>MATNFFIQPITEEAEAYYPPSVITNKRKDLGVDVYCCSDLVLQPGLNIVRLHIKVACEHMGKKCGFKIMARSSMCTHERLL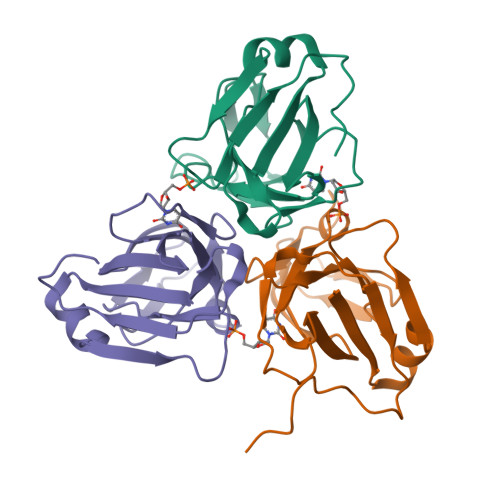ILANGIGLIDPGYVGELMLKIINLGDTPVQIWAKECLVQLVAQGDHVPDHINILKRNQIFPLFAPTPRGEGRFGSTGEAGIMRTHHHHHH[3x]> SLNVESSMVSQRGSSGQPVPVSANYLPLKGNMDGVFKYAVGFNPPVEDIRSRSQLLNEHKELIGLTRVFDGSTLYVPKRICEQRLDLMSTRQTDGASIKVTISLVDSVKNRDVVQLMNVIFKRILRSLKLQRIGRDYYDANSPLEVPQHKMQLWPGYVTAINRHEGGLMLVLDVSHRVMKTDTALDFLYELYHFNQDKFREEAFKQLVGSVVLTRYNNRTYEIDDIAWDKNPRCAFQDHAGSQITFVDYYKRAYDLDITDLEQPLLIHRPKKKQRGKQDEGRKEVEEMVCLVPELCAMTGLTDAARSDFKVMKDLAVHTRVPPEKRAESFRKFIQRLNTTKEASELLHSWGLVLDSRMLDMQGRRLPPEKILFKHSSIVANMEADWSRECLKEHVISAVSLL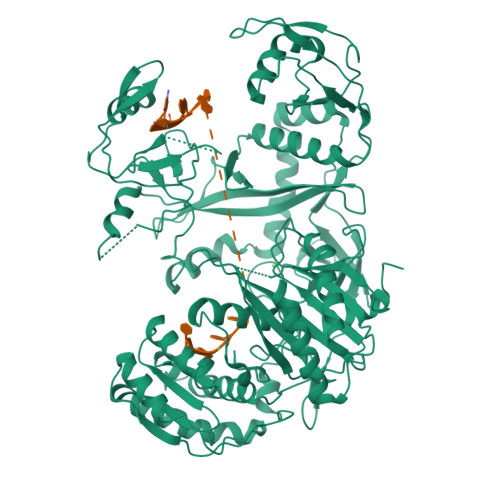DWAVLFVRKDQGKATDFVNMLSKVCPPIGMEVHEPKMVEVVNDRTESYLRALRELIAPRLQMVVIVFPTSRDDRYSAVKKLCCIESPIPSQVLIARTITQQQKLRSVAQKVALQMNAKLGGELWAVEIPLKSCMVVGIDVYHDKSYGNKSIAGFVASTNPSFTRWYSRTAMQEQSQELIHELKLCMQAALKKYNEMNQSLPERIIVFRDGVGEGREEYVSEFEVPQFNSCFSIFGENYCPKLAVVVVQKRITTRIFGRSGHSYDNPPPGVIVDHTITKSYDFYLVSQHVRQGTVSPTYYRVIYDKSGLKPDHLQRLTYKLTHMYYNWPGTIRTPAPCNYAHKLAFLVGKSLHRDPAHELSDRLFFL> MTGAVCPGSFDPVTLGHVDIFERAAAQFDEVVVAILVNPAKTGMFDLDERIAMVKESTTHLP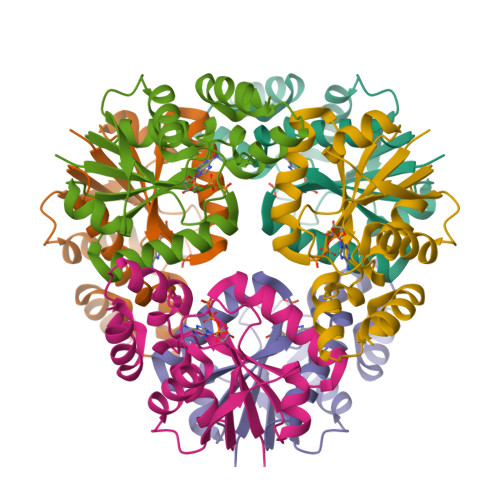NLRVQVGHGLVVDFVRSCGMTAIVKGLRTGTDFEYELQMAQMNKHIAGVDTFFVATAPRYSFVSSSLAKEVAMLGGDVSELLPEPVNRRLRDRLN> MNLMTTITGVVLAGGKARRMGGVDKGLLELNGKPLWQHVADALMTQLSHVVVNANRHQEIYQASGLKVIEDSLADYPGPLAGMLSVMQQEAGEWFLFCPCDTPYIPPDLAARLNHQRKDAPVVWVHDGERDHPTIALVNRAIEPLLLEYLQAGERRVMVFMRLAGGHAVDFSDH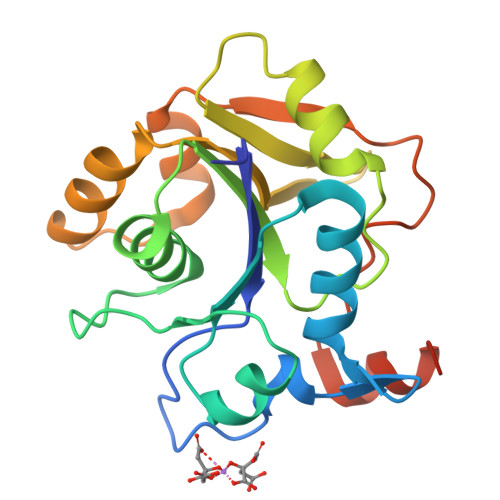KDAFVDVNTPEELARWQEKRSHHHHHH>MKKIAVFTGTRAEYGLLYWLMRDIQQDPELELQILATAMHYSPEHGETWKTIVKDGFEITESVEMLLSSDTSSAVVKSMGVGLLGFADALKRMQPDVLVVLGDRFEALAVTQAALIMHVPVAHLHGGEITEGAYDESIRHAITKMSNIHFAAAEEYKKRIIQLGEQPERVFNVGALGLDHIQRTTFKSISELSELYDFDFSKPYFLITYHPETNLLEENVAPLFDALKQINDVNFIFSYPNADNGNTNIVKAMLDLKAQLPDRVLLVKSFGIQNYLSVLKNALA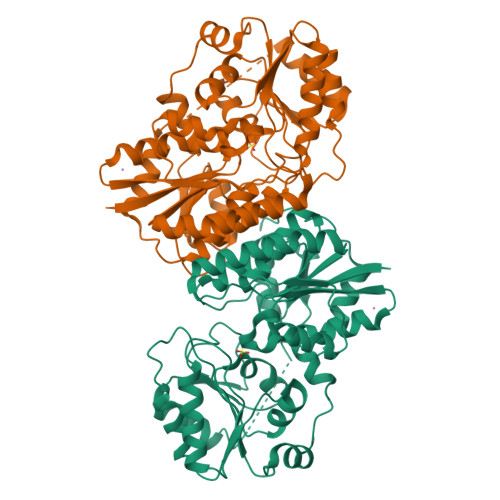MVGNSSSGLSEAPALQVPTVNIGDRQKGRLRCESILDVRLDENEIVEALQKAINFPKDQLSQVVPPLGLGNTSQKIIEVIKTTDFKKKAPFYDLLE[2x]>[4x]MGQGDESERIVINVGGTRHQTHRSTLRTLPGTRLAWLAEPDAHSHFDYDPRADEFFFDRHPGVFAHILNYYRTGKLHCPADVCGPLYEEELAFWGIDETDVEPCCWMTYRQHRDAEEALDSFGGAPLDNSADDADADGPGDSGDGEDELEMTKRLALSDSPDGRPGGFWRRWQPRIWALFEDPYSSRYARYVAFASLFFILVSITTFCLETHERFNPIVNKTEIENVRNGTQVRYYREAETEAFLTYIEGVCVVWFTFEFLMRVIFCPNKVEFIKNSLNIIDFVAILPFYLEVGLSGLSSKAAKDVLGFLRVVRFVRILRIFKLTR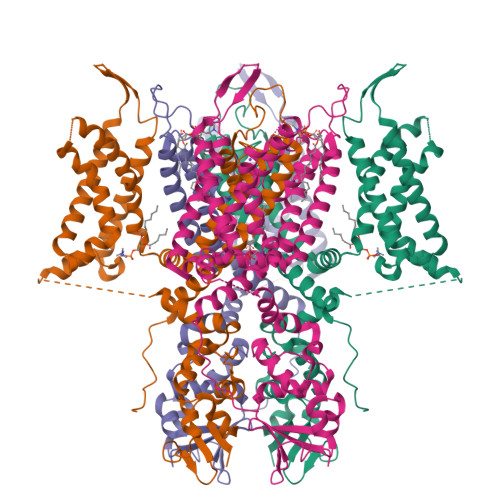HFVGLRVLGHTLRASTNEFLLLIIFLALGVLIFATMIYYAERIGAQPNDPSASEHTHFKNIPIGFWWAVVTMTTLGYGDMYPQTWSGMLVGALCALAGVLTIAMPVPVIVNNFGMYYSLAMAKQKLPKKKKKHIPRPPQLGSPNYCKSVVNSPHHSTQSDTCPLAQEEILEINRAGRKPLRGMSIAENLYFQ> METPEPRTTRTILVYMMANNSLNSFASKNIESMIEGATSKNLNGGNLIVYYAPAGSPPELLRIKEENGVVKKIHLKDYEKQNSADPDVMRSVIGEVVS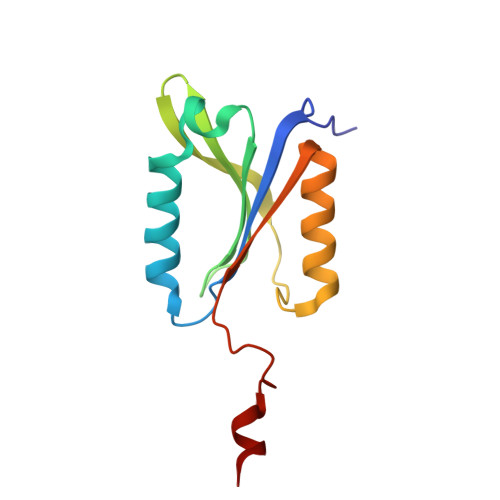QYPADSYGLVLWSHGTAWLPSDYQNKLK> APPKSVIRWCTISSPEEKKCNNLRDLTQQERISLTCVQKATYLDCIKAIANNEADAITLDGGQVFEAGLAPYKLKPIAAEVYEHTEGSTTSYYAVAVVKKGTEFTVNDLQGKTSCHTGLGRSAGWNIPIGTLLHRGAIEWEGIESGSVEQAVAKFFSASCVPGATIEQKLCRQCKGDPKTKCARNAPYSGYSGAFHCLKDGKGDVAFVKHTTVNENAPDQKDEYELLCLDGSRQPVDNYKTCNWARVAAHAVVARDDNKVEDIWSFLSKAQSDFGVDTK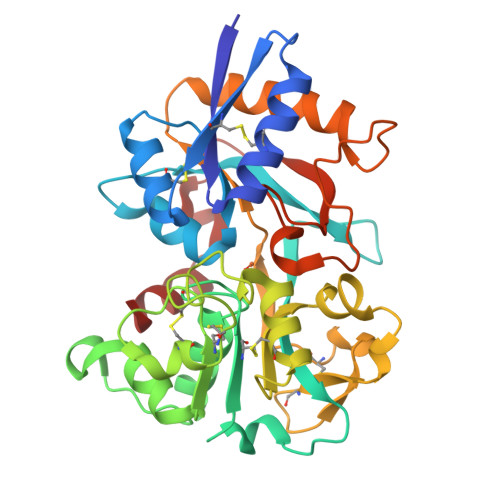SDFHLFGPPGKKDPVLKDLLFKDSAIMLKRVPSLMDSQLYLGFEYYSAIQSMR> MTGGMKPPARKPRILNSDGSSNITRLGLEKRGWLDDHYHDLLTVSWPVFITLITGLYLVTNALFALAYLAVGDVIENARPGSFTDAFFFSVQTMATIGYGKLIPIGPLANTLVTLEALVGMLGLAVAASLIYCRFCRPTAGVLFSSRMVISDFEGKPTLMMRLANLRIEQIIEADVHLVLVRSEISQEGMVFRRFHDLTLTRSRSPIFSLSWTVMHPIDHHSPIYGETDETLRNSHSEFLVLFTGHHEAFAQNVHARHAYSSDEIIWGGHFVDVFTTLPDGRRALDLGKFHEIAQHHHHHH

Potassium channels propagate electrical signals, maintain membrane potentials and facilitate numerous downstream cellular processes. KirBac3.1 adopts the canonical fold of a K+ channel, with inner and outer membrane-spanning helices supporting an inclined, shorter, pore helix that supports the signature selectivity filter. All feature an hourglass-like constriction at the intracellular opening, leading to the widespread conclusion that the canonical permeation gate at the helix bundle crossing is closed (or nearly so) in all Kir structures, whether determined by crystallography or single-particle cryo-EM. Thus, data presented here indicate that inward rectifiers (Kir) are able to conduct without requiring the substantial conformational changes predicted by the canonical gating mechanism.

To covalently constrain the dimensions of the hourglass-like constriction, paired cysteine point mutants were introduced into KirBac3.1 upon a cysteine-less background, in which each of the three native cysteine residues were substituted for serine or valine (C262S, C71V, C119V). This allowed us to covalently link the four inner helices into a tetramer without obstructing the conduction pathway. Following purification of A133C-T136C and S129C-F135C, covalent linkages between adjacent subunits were generated, either by direct disulfide formation using Cu2+ as the oxidant or by the crosslinking reagents 1,1-methanediyl bismethanethiosulfonate (MTS-1-MTS), which forms compact linkages (CysS–S–CH2–S–SCys) with slightly more tolerance than direct disulfides (CysS–SCys), and dibromobimane, a rigid bicyclic molecule. To visually inspect the channels for intact crosslinks or unanticipated effects on structure, crystal structures of two of the KirBac3.1 adducts, S129C-F135C-MTS-1-MTS and A133C-T136C-bimane were determined. In both mutants, four crosslinks encircle the conduction pathway at the Tyr132 as anticipated. Both revealed electron density bridging between adjacent inner helices, consistent with the predicted covalent linkages. An overlay of both crosslinked structures onto the native pore is illustrated. The cysteine-pair mutants were assayed under identical experimental conditions to wild type. All eight variants of the S129C-F135C or A133C-T136C mutants, either with reduced cysteine sulfhydryl moieties or as covalently-linked adducts with inner helices tethered at Tyr132, mediated K+ movement out of liposomes, with no significant difference in signal from wild type in any of the crosslinked populations, indicating that crosslinking did not prevent K+ flux through the Kir channels. The differences in rate (and overall signal) between crosslinked and reduced forms of the pore are not significant, which indicates the enforced constriction is not rate limiting.> MFENITAAPADPILGLADLFRADERPGKINLGIGVYKDETGKTPVLTSVKKAEQYLLENETTKNYLGIDGIPEFGRCTQELLFGKGSALINDKRARTAQTPGGTGALRVAADFLAKNTSVKRVWVSNPSWPNHKSVFNSAGLEVREYAYYDAENHTLDFDALINSLNEAQAGDVVLFHGCCHNPTGIDPTLEQWQTLAQLSVEKGWLPLFDFAYQGFARGLEEDAEGLRAFAAMHKELIVASSYSKNFGLYNERVGACTLVAADSETVDRAFSQMKAAI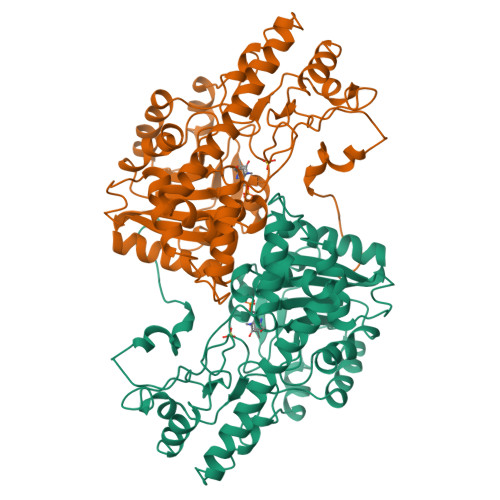DANYSNPPAHGASVVATILSNDALRAIWEQELTDMRQRIQRMRQLFVNTLQEKGANRDFSFIIKQNGMFSFSGLTKEQVLRLREEFGVYAVASGRVNVAGMTPDNMAPLCEAIVAVL>[4x]MAHHHHHHMLKLIVETKTLVQSLGFASSVVEKRNVIPEYANIKLSAQDGNLELSSTNMDLYLSQKIAVQVVSEGECTVSTKTLNDIVRKLPDSELTLTDLGTTGLEIKGKNCKFNLFTLPVSSFPAMDSINPEASFKISCTDFAKIIESTKFSISLDETRYNLNGVYLHIKDKEFCSASTDGHRLSISWVTLEKQIKNFGVILPQKS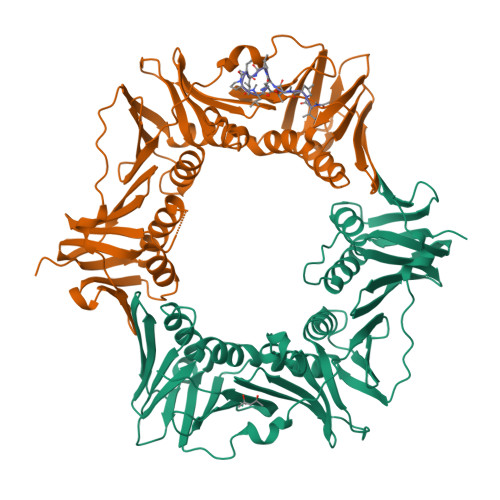AEEILKIVKDPKNINEDIEILLNSNKIKFICNENTIMLSKLIDGTFPDYSTFIPESSSSKLVINRKMFADSIERIAIITVEKFRAVKLSLSRETLEISAVGEARGNAKEVINSSQDKESFYEYNSDESLAIGFNPQYLEDVLKAVKSDLVELYFSDVSAPVLIKFPENPKDIFIVLPVKV;>[2x]XVPTLPLVPXG>[2x]MAHHHHHHVGTFENITAAPADPILGLADLFRADERPGKVDLGVGVYKDETGKTPVLTSVKKAEQYLLENETTKTYLGLDGLPEFGRCTQELLFGKGSALINDKRARTAQTPGGSGALRVAADFLAKNTSVKRVWVSNPSWPNHKAIFNSAGLEVREYAYYDAENHTLDFDALINSLNEAQAGDVVLFHGCCHNPTGADPTLEQWQTL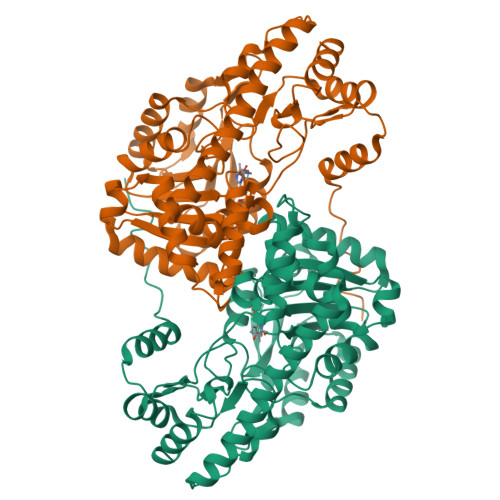AQLSVEKGWLPLIDIAYQGFGRGLEEDAEGLRAFAAMHKELIVASSCSKNFGLYNERVGACTLVAADSETVDRAFGQMKAAIRANYSNPPAHGASVVATILSNDALRAIWEQELTDMRQRIQRMRQLFVNTLQEKGANRDFSFVIKQNGMFSFSGLTKEQVLRLREEFGVYAVASGRVNVAGMTPDNMAPLCEAIVAVL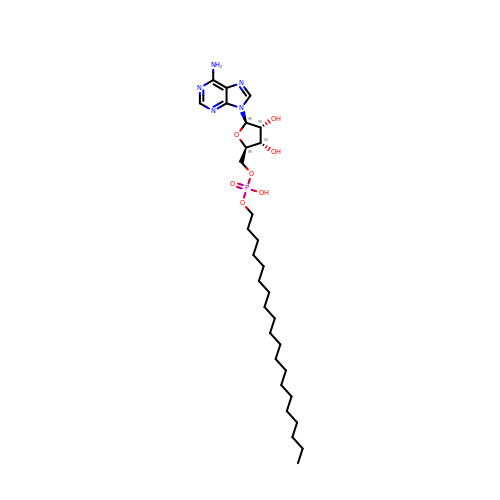[(2~{R},3~{S},4~{R},5~{R})-5-(6-aminopurin-9-yl)-3,4-bis(oxidanyl)oxolan-2-yl]methyl icosyl hydrogen phosphate | C30 H54 N5 O7 P | JFYKNVSLLXBVHG-BQOYKFDPSA-N> AAPVSEPTVARQKLLALLGQVQTYVFQIELLRRCDPHIGRGKLPQLKLNALQVRALRRRLRPGLEAQAGAFLTPLSVTLELLLEYAWREGERLLGSLETFATAGDVAAFFTETMGLARPCPYHQRVRLDTYGGTVHMELCFLHDVENFLKQLNYCHLITPSRGATAALERVREFMVGAVGSGLIVPPELSDPSHPCAVCFEELCVTANQGATIA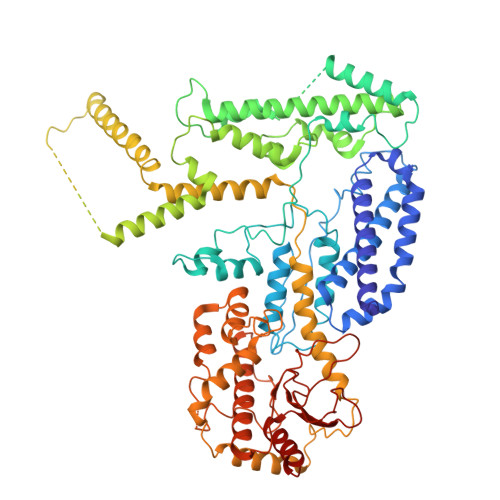SRLADRICNHVTQQAQVRLDANELRRYLPHAAGLSDADRARALSVLDHALARTAGGDGQPHPSPENDSVRKEADALLEAHDVFQATTPGLYAISELQFWLASGDRAGQTTMDAFASNLTALARRELQQETAAVAVELALFGRRAEHFDRAFGSHLAALDMVDALIIGGQATSPDDQIEALIRACYDHHLTTPLLRRLVSPEQCDEEALRRVLARMGAGGAADAPKGGAGPDDDGDRVAVEEGARGLGAPGGGGEDEDRRRGPGGQGPETWGDIATQAAADVRERRRLYADRLTKRSLASLGRCVREQRGELEKMLRVSVHGEVLPATFAAVANGFAARARFCALTAGAGTVIDNRSAPGVFDAHRFMRASLLRHQVDPALLPSITHRFFELVNGPLFDHSTHSFAQPPNTALYYSVENVGLLPHLKEELARFIMGAGGSGADWAVSEFQRFYCFDGISGITPTQRAAWRYIRELIIATTLFASVYRCGELELRRPDCSRPTSEGRYRYPPGVYLTYDSDCPLVAIVESAPDGCIGPRSVVVYDRDVFSILYSVLQHLAPR> MSSKYAVKLKTDFDNPRWIKRHKHMFDFLDINGNGKITLDEIVSKASDDICAKLEATPEQTKRHQVCVEAFFRGCGMEYGKEIAFPQFLDGFKQLATSELKKWARNEPTLIREWGDAVFDIFDKDGSGTITLDEWKAYGKISGISPSQEDC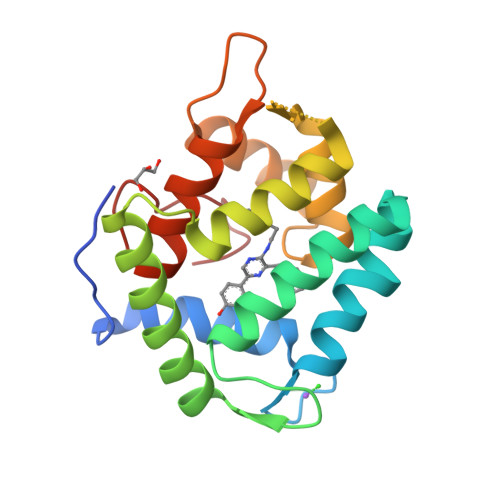EATFRHCDLDNSGDLDVDEMTRQHLGFWYTLDPEADGLYGNGVP>[4x]MDLSGKMVKQVEILSDGIVFYEIFR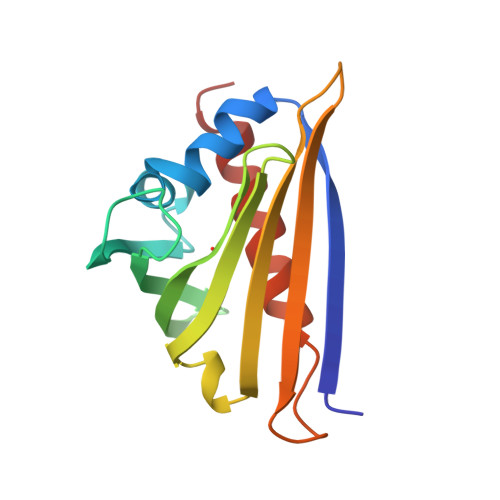YRLYLISEMSPVNIQGVDLLEGNWGTVGSVIFFKYTIDGKEKTAKDIVEAIDEETKSVTFKIVEGDLMELYKTFIIIVQVDTKGEHNSVTWTFHYEKLKEDVEEPNTLMNFCIEITKDIETYHLK>MGQIFSRSASPIPRPPRGLAAHHWLNFLQAAYRLEPGPSSYDFHQLKKFLKIALETPARICPINYSLLASLLPKGYPGRVNEILHILIQTQAQIPSRPAPPPPSSPTHDPPDSDPQIPPPYVEPTAPQVLPVMHPHGAPPNHRPWQMKDLQAIKQEVSQAAPGSPQFMQTIRLAVQQFDPTAKDLQDLLQYLCSSLVA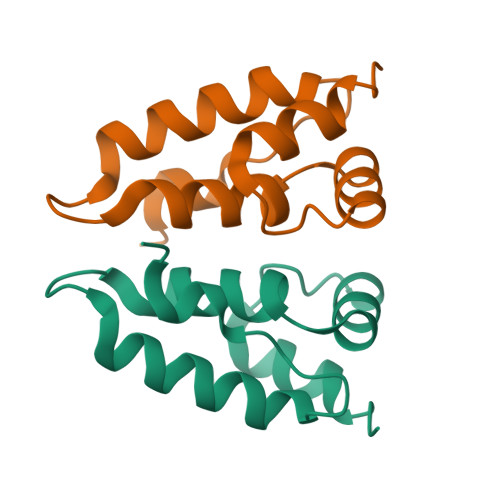SLHHQQLDSLISEAETRGITGYNPLAGPLRVQANNPQQQGLRREYQQLWLAAFAALPGSAKDPSWASILQGLEEPYHAFVERLNIALDNGLPEGTPKDPILRSLAYSNANKECQKLLQARGHTNSPLGDMLRACQTWTPKDKTKVLVVQPKKPPPNQPCFRCGKAGHWSRDCTQPRPPPGPCPLCQDPTHWKRDCPRLKPTIPEPEPEEDALLLDLPADIPHPKNSIGGEV[2x]>[2x]MGSHHHHHHSSGLVPRGSHMNQSSLLAEFGDPITRVENALQAL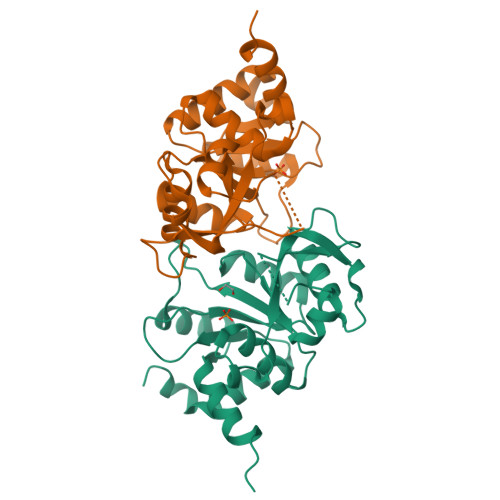REGRGVLLLDDEDRENEGDIIYAVESLTTAQMALMIRECSGIVCLCLTEAQADRLALPPMVVNNNSANQTAFTVSIEAKHGVTTGVSAQDRVTTIKTAANPQAKPEDLARPGHVFPLRARAGGVLARRGHTEGTVDLMQMAGLQPAGVLCELTNPDGSMAKTPEIIEFGKLHNMPVLTIEDMVQYRIQFDLKLA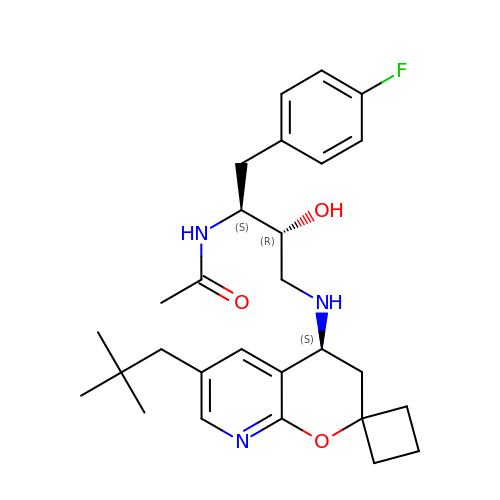N-((2S,3R)-1-(4-fluorophenyl)-3-hydroxy-4-((6'-neopentyl-3',4'-dihydrospiro[cyclobutane-1,2'-pyrano[2,3-b]pyridin]-4'-yl)amino)butan-2-yl)acetamide | C28 H38 F N3 O3 | FBJQDUYQPYABBR-CCDWMCETSA-N> GPEFEAAACKKYMSKLRTIVAAQSRFLSTYDGAENLCLEDIYTENTLEVRTEVGMAGPLHKSPAALGLEELFSPNGHLNEDADTVLVVGEAGSGKSTLLQQVHLLWATGQDFQEFLFVFPFSCRQLQCVARPLSVMTLLFEHCCWPDVGQQDVFQFLLDHPDRILLTFDGFDEFKFKFTDHERHCSPTDPTSVQTLLFNLLQGNLLKNARKVLTSRPDAVSAFLRKYVRTEFNLKGFSEEGIELYLRKCHREPGVADRLIHLLQTTSALHGLCHLPVFSWMVSKCHQELLLQDGGSPKTTTDMYLLILQHFLRHASLPDSASQGLGPSLLQGRLPTLLRLGQLALWGLGMCCYVFSAQQLQAAQVDPDDISLGFLVQAQGVVPGSTAPLEFLHITFQCFLAAFYLVLSTDVPTASLRYLFNCRRPGSSPLSRLLPRLCVQGSEHKESTVAALLQKTEPHNLQITAAFLAGLLSREHRDLLAACQASERSLLRRRACARWCLARSLHKHFRSIPPAVPGEAKSMHAMPGFLWLIRSLYEMQEERLAQEAVRGLNVEHLKLTFCGVGPAECAALAFVLRHLRRPVALQLDHNSVGDIGVEQLLPCLGACKALYLRDNNISDRGICKLIEHALHCEQLQKLALFNNKLTDGCAHSVAQLLACKQNFLALRLGNNHITAEGAQVLAEGLRDNSSLQFLGFWGNKVGDKGAQALAEALSDHQSLKWLSLVGNNIGSVGAQALASMLEKNVALEELCLAANHLQDAGVCSLAEGLKRNSSLKVLKLSNNCITFVGAEALLQALASNDTILEVWLRGNPFSPEEMEALSHRDSRLLL

NOD2, also known as NLRC2 or CARD15, belongs to the NLRC subfamily of NLRs. NOD2 possesses two tandem CARDs that function as an effector domain and is activated by muramyl dipeptide (MDP), a bacterial cell wall fragment9101112. On activation by MDP, NOD2 is believed to undergo self-oligomerization via the central NOD domain, providing a scaffold for recruiting RIPK2 (receptor-interacting serine–threonine kinase 2) through CARD–CARD interactions. Here, we determined the crystal structure of the inactive ADP-bound form of NOD2, and revealed that ADP-bound NOD2 is maintained in an auto-inhibited/closed form through ADP-mediated and inner domain interactions of the NOD domain.

Moreover, we introduced surface entropy reduction (SER) mutations (E943A, E944A, K635A, E636A, E709A and K711A) into the OcNOD2ΔCARD construct to produce the OcNOD2ΔCARDSER construct. These CARD-defective NOD2 proteins for structural study would be inactive, because the CARD domain is required for triggering NF-κB activation through the serine–threonine kinase RIPK2. The OcNOD2Δloop construct exhibited activity comparable to the wild-type OcNOD2 in response to MDP, while the OcNOD2SER construct exhibited no activity in NF-κB reporter assays in HEK293T cells. Gel filtration chromatography analyses revealed that full-length OcNOD2, OcNOD2ΔCARD, OcNOD2ΔCARDΔloop and OcNOD2ΔCARDSER exist as monomers in solution. In addition, we determined the structure of OcNOD2ΔCARDSER, which is isomorphous to the form 1 of OcNOD2ΔCARDΔloop crystal, at 3.1 Å resolution. The structures of the NOD2 molecules in these crystals were essentially the same, with root mean squared deviations (r.m.s.d.) between 0.4 and 1.1 Å. Of note, several mutated residues for SER mapped to HD2. Mutation of these residues may alter the charge distribution, resulting in reduction of the activity of OcNOD2ΔCARDSER.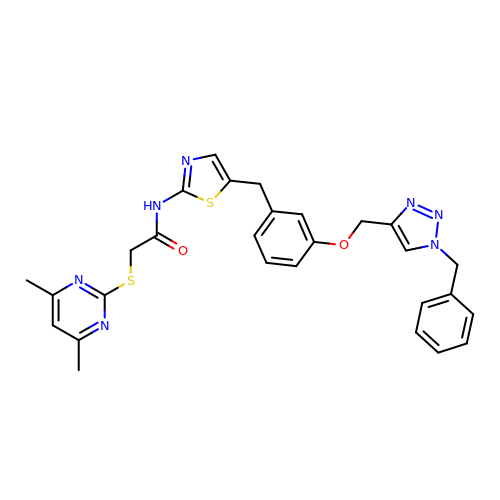N-(5-{3-[(1-benzyl-1H-1,2,3-triazol-4-yl)methoxy]benzyl}-1,3-thiazol-2-yl)-2-[(4,6-dimethylpyrimidin-2-yl)sulfanyl]acetamide | C28 H27 N7 O2 S2 | YWLNYZXFIAFWSF-UHFFFAOYSA-N>METDNVELAQSKRKVVLAEQGSFYIGGRTVTGPGKFDPSKPVIPYSNEGATFYINQMYVNFQAPVRPRGLPLVFWHGGGLTGHIWESTPDGRPGFQTLFVQDRHTVYTIDQPGRGRGNIPTFNGPFGQLEEESIVNTVTGNSSKEGAWVRDRLGPAPGQFFENSQFPRGYEDNYFKEMGFSPSISSDEIVDAVVKLVTHIGPCVLVTHAASGVLGMRVATHAKNVRGIVAYEPATSIFPKGKVPEIPPLADKKSQIFPPFEIQESYFKKLAKIPIQFVFGDNIPKNPKSAYWFLDWWRVTRYAHSL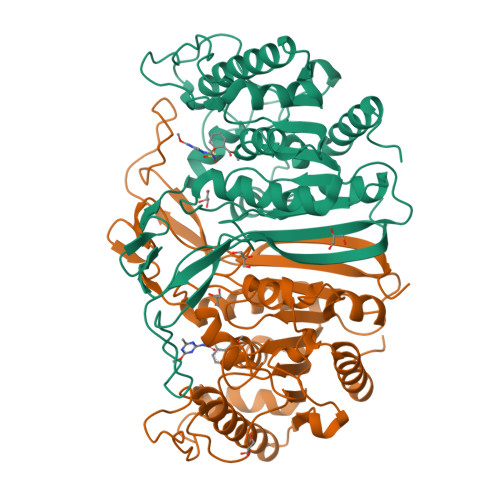SLEAINKLGGQASLLDLPTAGLRGNTHFPFTDRNNVQVASLLSDFLGKHGLDQNESLEHHHHHH[2x]> KNNDKLTLWTTPAPSPNCRLNAEKDAKLTLVLTKCGSQILATVS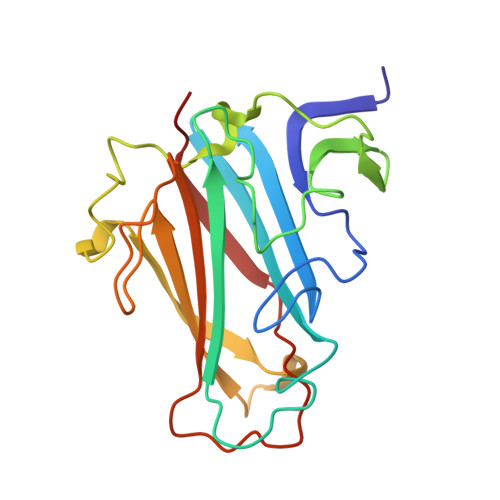VLAVKGSLAPISGTVQSAHLIIRFDENGVLLNNSFLDPEYWNFRNGDLTEGTAYTNAVGFMPNLSAYPKSHGKTAKSNIVSQVYLNGDKTKPVTLTITLNGTQETGDTTPSAYSMSFSWDWSGHNYINEIFATSSYTFSYIAQE>MVMSDPVSYTRKDSIAVISMDDGKVNALGPAMQQALNAAIDNADRDDVGALVIT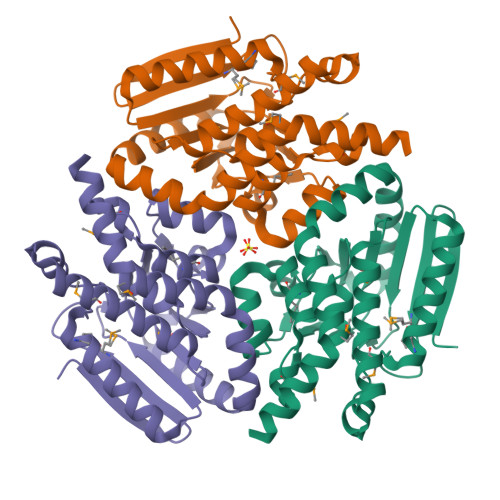GNGRVFSGGFDLKILTSGEVQPAIDMLRGGFELAYRLLSYPKPVVMACTGHAIAMGAFLLSCGDHRVAAHAYNIQANEVAIGMTIPYAALEIMKLRLTRSAYQQATGLAKTFFGETALAAGFIDEIALPEVVVSRAEEAAREFAGLNQHAHAATKLRSRADALTAIRAGIDGIAAEFGLAENLYFQSHHHHHHWSHPQFEK[2x]> GSSAPRFLTRPKAFVVSVGKDATLSCQIVGNPTPQVSWEKDQQPVAAGARFRLAQDGDLYRLTILDLALGDSGQYVCRARNAIGEAFAAVGLQVDAEA;> GSSRGIPPKIEALPSDISIDEGKVLTVACAFTGEPTPEVTWSCGGRKIHSQEQGRFHIENTDDLTTLIIMDVQKQDGGLYT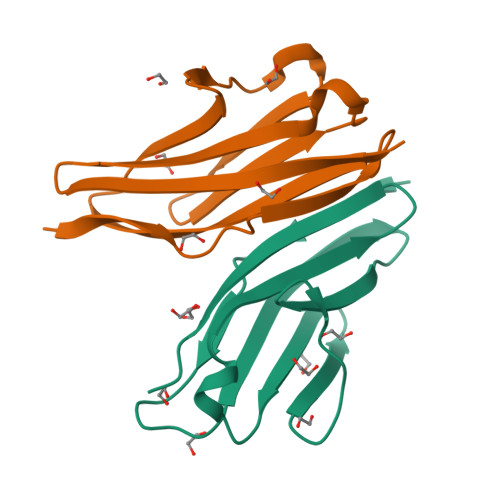LSLGNEFGSDSATVNIHIRSI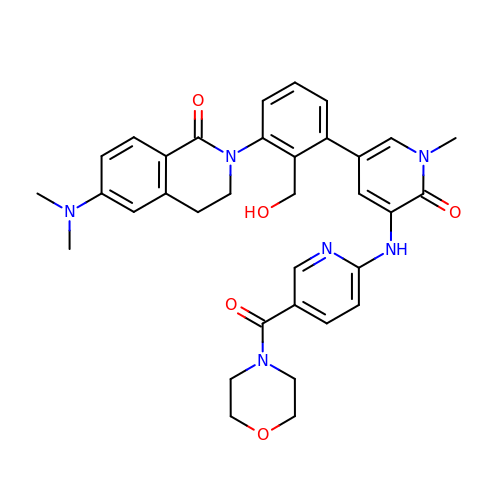6-(dimethylamino)-2-[2-(hydroxymethyl)-3-(1-methyl-5-{[5-(morpholin-4-ylcarbonyl)pyridin-2-yl]amino}-6-oxo-1,6-dihydropyridin-3-yl)phenyl]-3,4-dihydroisoquinolin-1(2H)-one | C34 H36 N6 O5 | SJBGHIGDLWCJIO-UHFFFAOYSA-N>APKCIECHINIEMDPVLHDVFKLQVCKQCSKEHPEKYALLTKTECKEDYFLTDPELNDEDLFHRLEKPNPHSGTFARMQLFVRCEVEAFAFKK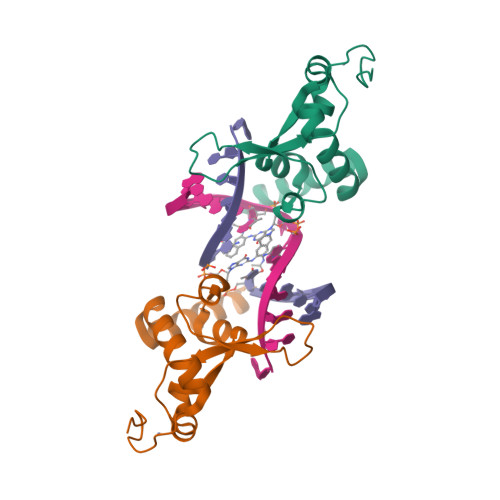WGGEEGLDEEWQRREEGKAHRREKKY[2x]>HHHHHHMEPACKYDFATSVLFTEAELHTRMRGVAQRIADDYSNCNLKPLENPLVIVSVLKGSFVFTADMVRILGDFGVPTRVEFLRASSYGHDTKSCGRVDVKADGLCDIRGKHVLVLEDILDTALTLREVVDSLKKSEPASIKTLVAIDKPGGRKIPFTAEYVVADVPNVFVVGYGLD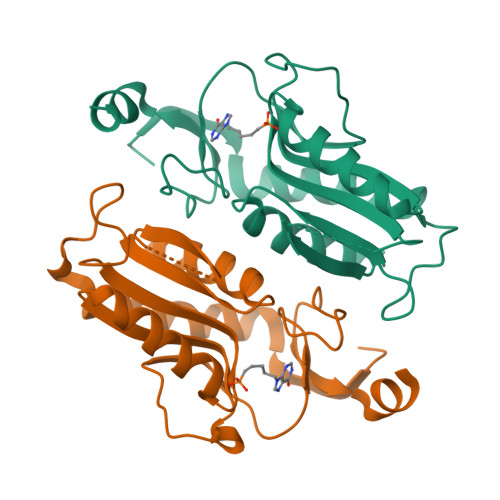YDQSYREVRDVVILKPSVYETWGKELERRKAAGEAKR[4x]> GPMRTKIVVKVHMPCGKSRAKAMALAASVNGVDSVEITGDDKDRLQVVGRGIDPVRLVALLREKCGLAELLQVEEVKE;> GPMRAIDLSRERDPNFFDNADIPVPECFWFMFKNNVRQDAGTCYSSWKMDKKVGPNWVHIKSDDNCNLSGDFPPGWIVLGKKRPGF

Nucleotide-binding leucine-rich repeat (NLRs) receptors are intracellular immune proteins that trigger robust defense responses upon recognition of pathogen virulence proteins (effectors) delivered into the host during infection. One such mechanism is the use of integrated domains, which function as effector baits embedded within the canonical NLR architecture. The RGA5/RGA4 and Pik pairs harbor an integrated heavy metal-associated (HMA) domain in their sensor NLRs RGA5 and Pik-1 that directly bind and recognize MAX (Magnaporthe oryzae avirulence and ToxB like) effectors. The HMA domains of Pik-1 and RGA5 use spatially distinct protein interfaces for effector recognition (De la Concepcion et al. 2018; De la Concepcion, Maidment, et al. 2021; Guo et al. 2018; Varden et al. 2019).

Using a host target of AVR-Pik, O. sativa heavy metal-associated isoprenylated plant protein 19 (OsHIPP19) as a structural template for APB, we generated an RGA5 variant, termed the APB mutant. The APB mutant contains the point mutations Glu1033Asp, Val1039Gln, Met1065Gln, Leu1068Glu, Glu1070Lys, and Lys1071Glu that localize to a potential APB interface of the RGA5 HMA. As the effector recognition interfaces of RGA5 and Pikm-1 HMA domains are different, we determined a crystal structure of the complex between the APB mutant and AVR-PikF, to validate our structural modeling of the RGA5 HMA and confirm we had engineered an AVR-Pik/Pik-HMA-like interface into RGA5 HMA. Following this, we used a coexpression approach to purify an APB/AVR-PikF complex, which was used to obtain crystals via sparse matrix screening. X-ray diffraction data were collected at the Diamond Light Source, Oxford, resulting in a 1.3-Å data set (see details of crystallization and structure solution in Materials and methods). The APB/AVR-PikF complex shares the same interface as Pikm-1 HMA/AVR-PikD and OsHIPP19/AVR-PikF complexes. Structural alignment of these complexes results in an RMSD of 0.51 and 0.39 Å, respectively. As predicted, each of the 6 mutations in the RGA5 HMA generated to facilitate APB is located at the effector interface. Therefore, to quantify the affinity between the APB and AVR-Pik effectors, we used single-cycle kinetics with a long dissociation phase, which allowed us to calculate a KD of 0.31, 2.95, and 16.50 nM for AVR-PikD, AVR-PikC, and AVR-PikF respectively.>[2x]AFYKREMFDPAEKYKMDHRRRGIALIFNHERFFWHLTLPERRGTCADRDNLTRRFSD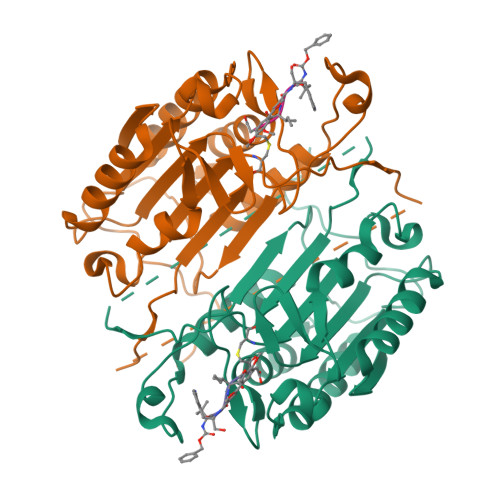LGFEVKCFNDLKAEELLLKIHEVSTVSHADADCFVCVFLSHGEGNHIYAYDAKIEIQTLTGLFKGDKCHSLVGKPKIFIIQACRGNQHDVPVIPLDVVDAASVYTLPAGADFLMCYSVAEGYYSHRETVNGSWYIQDLCEMLGKYGSSLEFTELLTLVNRKVSQRRVDFCKDPSAIGKKQVPCFASMLTKKLHFFPKSNGNSHHHHHH> MASHKKTESNQIIKTFSFKIKNANGLSLDVLNDAITEYQNYYNICSDWIKDHLTMKISELYKYIPNEKKNSGYALTLISDEWKDKPMYMMFKKGYPANNRDNAIYETLNTCNTEHYTGNILNFSDTYYRRFGYVASAISNYVTKISKMSTGSRSKNISNDSDVDTIMEQVIYEMEHNGWTSVKDWENQMEYLESKTDSNPNFVYRMTTLYEFYKSHIDEVNSKMETMSIDSLIKFGGCRRKDSKKSMYIMGGSNTPFDITQIGGNSLNIKFSKNLNV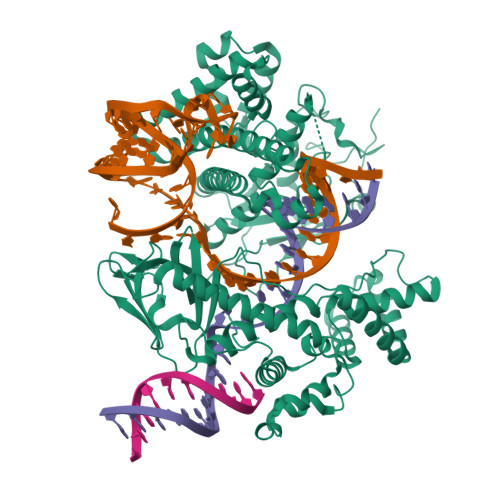DVFGRYDVIKDNTLLVDIINGHGASFVLKIINDEIYIDINVSVPFDKKIATTNKVVGIDVNIKHMLLATNILDDGNVKGYVNIYKEVINDSDFKKVCNSTVMQYFTDFSKFVTFCPLEFDFLFSRVCNQKGIYNDNSAMEKSFSDVLNKLKWNFIETGDNTKRIYIENVMKLRSQMKAYAIVKNAYYKQQSEYDFGKSEEFIQEHPFSNTDKGIEILNKLDNISKKILGCRNNIIQYSYNLFEINGYDMVSLEKLTSSQFKKKPFPTVNSLLKYHKILGCTQEEMEKKDIYSVIKKGYYDIIFDNDVVTDAKLSAKGELSKFKDDFFNLMIKSIHFADIKDYFITLSNNGTAGVSLVPSYFTSQMDSIDHKIYFVQDNKSGKLKLANKHKVRSSQEKHINGLNADYNAARNIAYIMENTDCRNMFMKQSRTDKSLYNKPSYETFIKTQGSAVAKLKKEGFVKILDEASVGSSGHHHHHH>MTRAERKRQHINHALSIGQKRETGLDDITFVHVSLPDLALEQVDI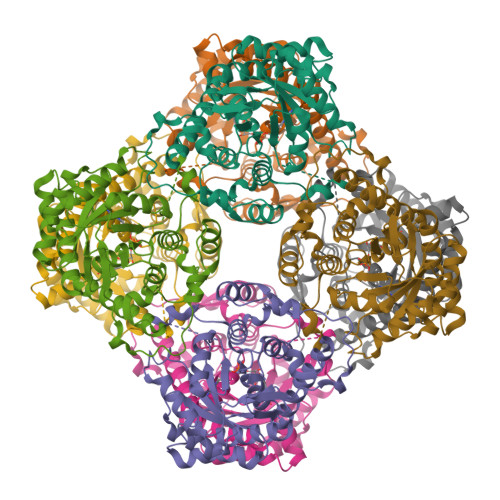STKIGELSSSSPIFINAMTGGGGKLTYEINKSLARAASQAGIPLAVGSQMSALKDPSERLSYEIVRKENPNGLIFANLGSEATAAQAKEAVEMIGANALQIHLNVIQEIVMPEGDRSFSGALKRIEQICSRVSVPVIVKEVGFGMSKASAGKLYEAGAAAVDIGGYGGTNFSKIENLRRQRQISFFNSWGISTAASLAEIRSEFPASTMIASGGLQDALDVAKAIALGASCTGMAGHFLKALTDSGEEGLLEEIQLILEELKLIMTVLGARTIADLQKAPLVIKGETHHWLTERGVNTSSYSVR[2x]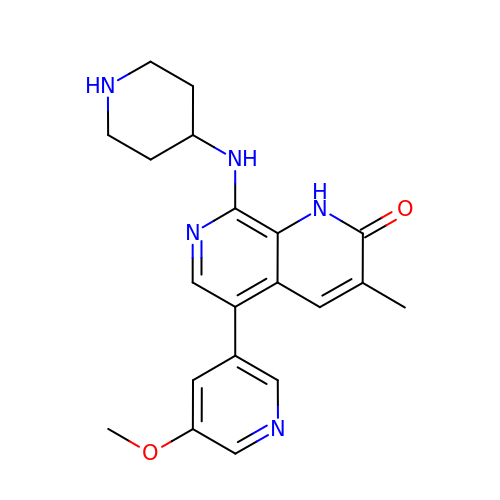5-(5-methoxypyridin-3-yl)-3-methyl-8-[(piperidin-4-yl)amino]-1,2-dihydro-1,7-naphthyridin-2-one | C20 H23 N5 O2 | FPQQERRFPULCIK-UHFFFAOYSA-N2-azanyl-~{N}-[2-(4-fluoranyl-3-oxidanyl-phenyl)carbonylquinolin-7-yl]ethanamide 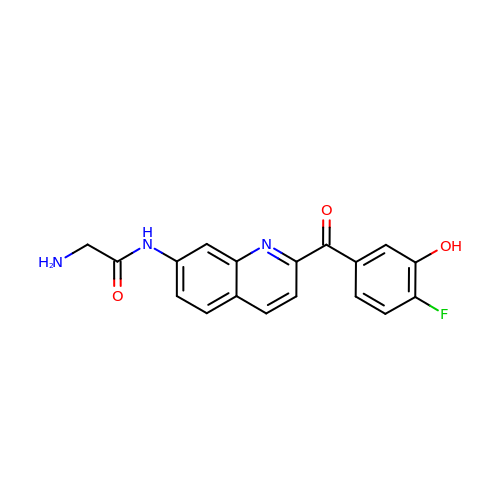| C18 H14 F N3 O3 | HEOXKDDZAJDQPA-UHFFFAOYSA-N>MRSSHHHHHHSSGLVPRGSHMESKKDDTDLKLVSHNVYMLSTVLYPNWGQYKRADLIGQSSYIKNNDVVIFNEAFDNGASDKLLSNVKKEYPYQTPVLGRSQSGWDKTEGSYSSTVAEDGGVAIVSKYPIKEKIQHVFKSGCGFDNDSNKGFVYTKIEKNGKNVHVIGTHTQSEDSRCGAGHDRKIRAEQMKEISDFVKKKNIPKDETVYIGGDLNVNKGTPEFKDMLKNLNVNDVLYAGHNSTWDPQSNSIAKYNYPNG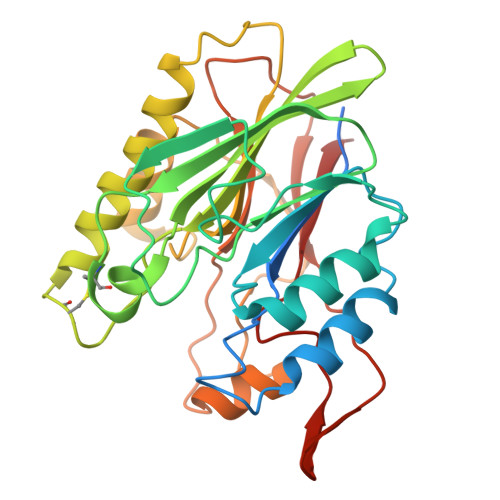KPEHLDYIFTDKDHKQPKQLVNEVVTEKPKPWDVDGYVYNDFSDHYPIKAYSK[4x]> MSFHITPTAAARDSETKQIDHNDSIRASYMTIEELHDAGAALSRDGADSLPGFMEFDFFERHRENEKEILRVYRTTAVDAENGATITPAAEWLLDNHYVIEEAIQEVRRDFPRKFYRQLPTMTVGGVTIPRVMALGWLYVAHTHSTVSRENMTALVDGYQTSQTLQIGELWALPSIIRFVLIENLRRISIRVERSRRMRQKANEVVDEIIRLNDAEASAALLKQVDSLVDDPTFATQFLYRLRNGSQTSGFAVAWLEERLHAAGTDAENVMMSEHNRLASGNVTMGNIVKSLREIDDTEWSVWFEEVSHIDKVLREETDYEILDFGSRNTYRNTIELLARRSPRTEVEVARAAVEMARSDLPAGADENHRVNVGSVLVGQRRFELEKALGYRPL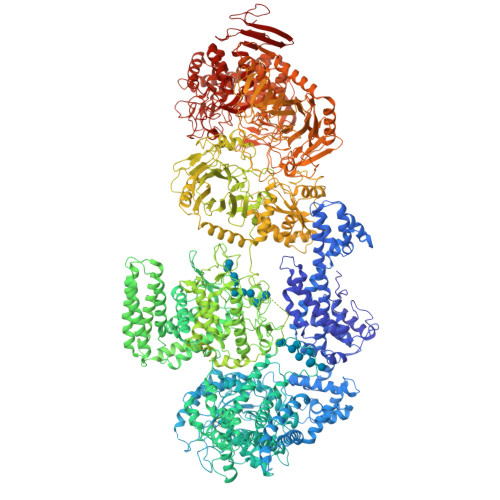ASQHIVRSMRKFNWLAIAAPVLLITAVAMLAVGWFLAKAGMPWYVVTAFLLMFALPASEGATGLFNTLVTFFVKPFRLVGYEFKNGIPEDARTLVAVPCMLTSRDSVDEMMRNIEVHYLANPHGEIYFSLVSDWRDAPYEQSDEDLEILDYAKRELAALNSRYAFDGKTRFYLLHRRRIYNSAEECWMGWERKRGKLHELNMLLRGDKDTTFLGGSNIVPADVKYVMTLDADTRLMRDAVTKLVGKMHHPINRPKIDPVSGRVVEGYGLLQPRVTPSLTTGKDASVFQRVFSINRGIDPYVFTVSDVYQDLTSEGTFTGKGLYDVDAFEAALKGRIEENSILSHDLLEGSFARCALVTDVELVEDFPTRYEVEVSRQHRWARGDWQLLPFIIDRARGVTAIGRWKMVDNLRRSLTPIAWFFASILGWYFMDPLGALIWQILLIFSLFVAPTLSLLSGLVPRSTDIVPQAHFFTIWSEIRATNAQVALRIVFIADAACMMTDAIVRSLYRLLVSHKLMLEWRTAASMQSSAQGSIVDYYRQMWHAPVVAMLGLLFAALPGDNAFLIGIPFTLLWVLSPAVAWYVSQSAETEDRLFVSEHVSFELRKIARRTWRYYEAFVTPQENHLPPDNFQETPEPIVASRTSPTNIGVYLLSVISARQFGWISFADTLERIENTIQTVEKMEKHRGHLYNWYHTDTLQTLGPRYVSAVDSGNLAGHLIAVSSACRDWAEAPSAHLQGNLDGIGDVAGILRETLKALPDNRKTLRPLHRRLEERIIGFSNALASVKREHEFASIRVINLAVLARDIQKLATNVDHEVKSAQSAEVTRWAQLLVESCEAHISDSAIDLTNMEPLRQRLASLRDRSRNLAFSMDFTFLYRKDRRLLSIGYRVESKELDEACYDLLASECRLTSLFAIAKGDLPTEHWYRLGRQVVPIGAQGALVSWSGSMFEYLMPPLVMQERQGGILNQTNNLIVKEQMNHGRRLGTPWGISEAAFNARDHNMNYQYTNFGVPTLGLKRGLGQNAVIAPYASILASQYDPDGALENLDKLRKLGALGQYGFHDAVDFTPTRVPDGKVCAVVYNYYAHHHGMSIAAVANVAFDGVLRELFHSDPVIEAAELLLQEKAPREVPVMSAKYEPETPGKEQADLLRAEVRSIADPAVRDREVVFLSNGHYSTMLTSTGAGYSKWNGQAISRWKADPTDDRWGTFIFLRDTTNGQWWSATAEPRVIEGEKTKTIFTDDKAEFHKTIGDLQSVVECIVATEHDAEGRRITLLNVGSEDRYIEVTSYMEPVIASEDDDNAHPLFSRMFVQTEIGRRGDVIRAWRNRRSQNEPGTVIAHLAADNAGPSRPTEFETDRAKFIGRGRSLREAAAFDAGATLSSSDGFTLDPILSLRRTVRVPAGKKVSVIFWTIAAPSREEVDKAIDRYRHPDAFAHELVHAWTRTQVQMRHVGVTSQQAAAFQHLGRYLTYPDMHLRADSETLKTGLASQRALWPLAISGDFPIFSLRINDDMDMDIAREALSAHEYLRSRGVIFDLVIVNERAASYAQDMQHALDHISETQRRINPADGGRPHVFSVRRDLMDEETWSALLAASRVVLHVRNGKIVDQINRAVSLFAANRGPDGSSDAAQARLPVPAFPVAEPVEDAGDLDFWNGFGGFAKNGQEYVVRLNGGQSTPHPWINVISNENFGFHISAEGAGFSWSRNSRDYQLTPWTNDPVINRPGEAFYVADVETGKLYTPCAALSRDPEAMFETRHGLGYSILTGVADTLEVELTQTVDREKPVKFSQVIVRNKGSKSRRLKVYAYVEWVLGNNGQKSAPFILSRHDAGSNAIFASNPYSIDYSARTSFLTLDSEASGFTTSRREFIGRFGSAQAPQGIVAGAALSGTTEVDGDPCAALMQEIHLKPGEERHMTFILGDADNAEEAEALVKDVRQADFLSVLEESKKFWTGFTGQLQVSTPDAGFNHMVNNWLPYQALACRILARTAFYQSSGAFGFRDQLQDTLAFLLYQPDLARTQILRAAGRQFPEGDVQHWWLPLTGAGVRTTISDDVVWLAYAINQYVSATGDAAILDESIPFLKGPALMPGQHDAFFQPETSERSATLYEHAALALDLAIHRTGENGLPLILGGDWNDGMNRVGVGGKGTSVWLGWFLAGALRDFIEIAEKRGDTDRVGKWASHREKLRHVLETAGWDGSYYRRGYFDDGTPLGSASSEECQIDSLGQSWSVLSGEGEEGRSRQAMDAVMEHLVDEKTGIIRLFTPPFSRASHDPGYIKGYPPGVRENGGQYTHAATWVVLALAKQGRAQEAWNCFKLLNPVNHALDAASSETYRVEPYVVTADVYGEGAYAGRGGWSWYTGSAGWLYRAAVEGILGITRTDGKLHVSPSLPEDWSGFSIRITLDGKARDIAVSRKAGTADVSVSVDG>MVEIILSHLIFDQAYFSKVWPYMDSEYFESGPAKNTFKLIKSHVNEYHSVPSINALNVALENSSFTETEYSGVKTLISKLADSPEDHSWLVKETEKYVQQRAMFNATSKIIEIQTNAELPPEKRNKKMPDVGAIPDIMRQALSISFDSYVGHDWMDDYEARWLSYMNKARKVPFKLRILNKITKGGAETGTLNVLMAGVNVGKSLGLCSLAADYLQLGHNVLYISMEMAEEVCAKRIDANMLDVSLDDIDDGHISYAEYKGKMEKWREKSTLGRLIVKQYPTGGADANTFRSLLNELKLKKNFVPTIIIVDYLGICKSCRIRVYSENSYTTVKAIAEELRALAVETETVLWTAAQVGKQAWDSSDVNMSDIAESAGLPATADFMLAVIETEELAAAEQQLIKQIKSRYGDKNKWNKFLMGVQKGNQKWVEIEQDSTPTEVNEVAGSQQIQAEQNRYQRNESTRAQLDALANELKF[6x];> MSSIPWIDNEFAYRALAHLPKFTQVNNSSTFKLRFRCPVCGDSKTDQNKARGWYYGDNNEGNIHCYNCNYHAPIGIYLKEFEPDLYREYIFEIRKEKGKSRPIEKPKELPKQPEKKIIKSLPSCVRLDKLAEDHPIIKYVKARCIPKDKWKYLWFTTEWPKLVNSIAPGTYKKEISEPRLVIPIYNANGKAESFQGRALKKDAPQKYITIEAYPEATKIYGVERVKDGDVYVLEGPIDSLFIENGIAITGGQLDLEVVPFKDRRVWVLDNEPRHPDTIKRMTKLVDAGERVMFWDKSPWKSKDVNDMIRKEGATPEQIMEYMKNNIAQGLMAKMRLSKYAKI

The T4 bacteriophage gp41 helicase and gp61 primase assemble into a primosome to couple DNA unwinding with RNA primer synthesis for DNA replication. The domain architecture of the gp41 helicase resembles the bacterial DnaB helicase13,14 with an NTD and a RecA-like CTD that are connected by a linking helix (LH). The gp61 primase is composed of an N-terminal ZBD and a C-terminal RPD that are linked by an 18-residue flexible loop. Here we report a series of cryo-EM structures of T4 primosome assembly intermediates.

The primosome map 3-II shows the gp61 primase bound to the active, planar gp41 helicase hexamer. By classifying the primosome particles based on the gp61 primase regions and refining the entire primosome particles in each class, we obtained three primosome EM maps. The three primosome structures are similar, but not identical, to each other because of the asymmetry of the seam present in the gp41 helicase; they differ in the location of the two gp41 helicase dimers that bind the gp61 primase. The gp61 ZBD and RPD bind the gp41 helicase similarly in the three binding modes with the ZBD binding to the first N-terminal helical hairpin dimer and the RPD binding to the second helical hairpin dimer in a clockwise direction when viewed from the primase side of the primosome. One gp61 primase has two binding sites on the helicase hexamer: the gp61 ZBD binds to two NTDs of one gp41 dimer, and the gp61 RPD binds to two NTDs of a second gp41 dimer. The two NTDs of the third gp41 dimer are unoccupied. In each binding pose, the ssDNA 5′-end emerging from the gp41 helicase consistently passes between the gp61 ZBD and RPD domains. The poses are non-equivalent because of the asymmetric helicase structure due to the presence of a seam between subunits A and F. In our initial primosome structure, there was no density for the RNA primer, but the density for the ssDNA was present stretching from the gp61 ZBD to the N-terminal lobe (NTL) of the gp61 RPD; therefore, this structure may represent an ssDNA-scanning configuration of the primosome in search of a priming recognition sequence. We suggest this is a DNA-scanning mode of the primosome in which the primase ZBD scans the ssDNA sequence for a 5′-GTT or 5′-GCT primer start site29 (step i).>MLYHLFVNNQVKLQNDFKPESVAAIRSSAFNSKGGTTVFNFLSAGENILLHISIRPGENVIVFNSRLKNGAWGPEERIPYAEKFRPPNPSITVIDHGDRFQIRFDYGTSIYYNKRIKENAAAIAYNAENSLFSSPVTVDVHGL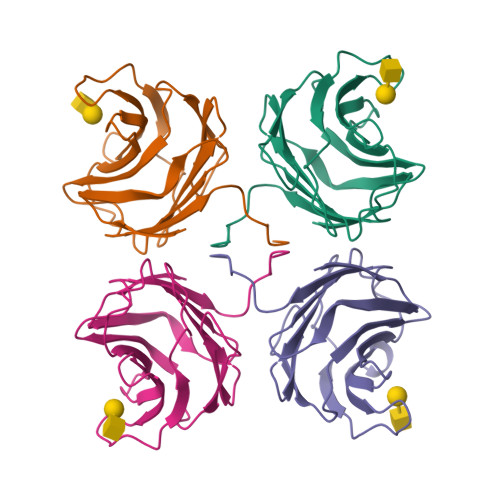LPPLPPA[4x]>GPLGSSTMGQVGRQLAIIGDDINRRYDSEFQTMLQHLQPTAENAYEYFTKIATSLFESGINWGRVVALLGFGYRLALHVYQH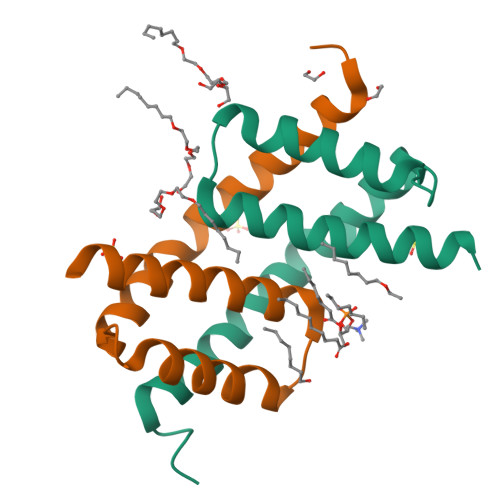GLT[4x]>SMPPHGELQYLGQIQHILRCGVRKDDRTGTGTLSVFGMQARYSLRDEFPLLTTKRVFWKGVLEELLWFIKGSTNAKELSSKGVKIWDANGSRDFLDSLGFSTREEGDLGPVYGFQWRHFGAEYRDMESDYSGQGVDQLQRVIDTIKTNPDDRRIIMCAWNPRDLPLMALPPC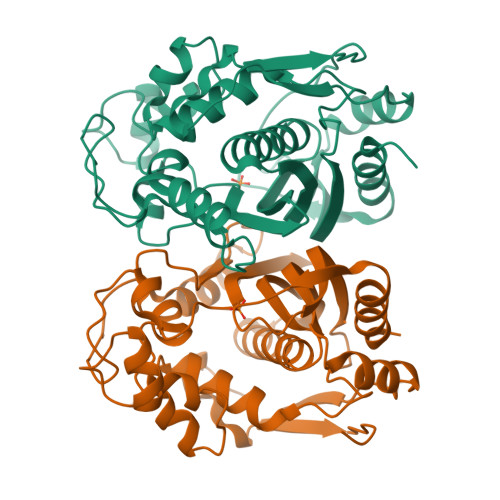HALCQFYVVNSELSCQLYQRSGDMGLGVPFNIASYALLTYMIAHITGLKPGDFIHTLGDAHIYLNHIEPLKIQLQREPRPFPKLRILRKVEKIDDFKAEDFQIEGYNPHPTIKMEMAV[6x]>MATNGMRPIHPGEILRDEFL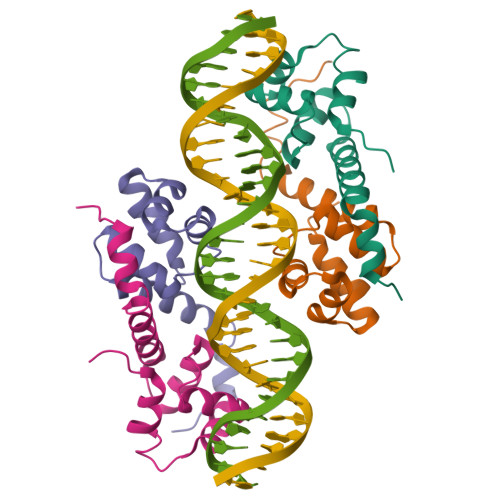MEFDISPAALARALKVSAPTVNDIVREQRGISADMAIRLGRYFDTSAQFWMNLQSEYSLATAYAANGKQIEHEIEPLLAHGGSHHHHHH[4x]>MAHHHHHHMSIIEFWLEAKATIDRLIEQFLNSNRDWDLVDISSYILKDGKRFRGTLNMFFTVALGGDIKDSYGGALAIEILHSASLALCDIVDLDATRRGDKAAWVVYGNRKVIFITNYLIPTALRIIQTSYGDDALNTSIELWKDTSVGALRDMYDNSDYIRTIELKTGSLFKLSTVLSAYASKHYNTKQQMLDVGKYLGIIYQVIDDFVDYKTKKVEEIDGSAKQLFKYYREGKLEEYVRSVYLEYKQKYDELISNIPFQSKYLSEIRSLPEFLANGLLKEANIDKI[2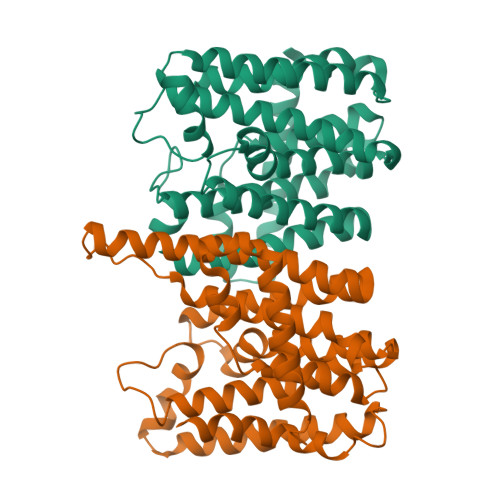x]>GSHMPAPHGGILQDLIARDALKKNELLSEAQSSDILVWNLTPRQLCDIELILNGGFSPLTGFLNENDYSSVVTDSRLADGTLWTIPITLDVDEAFANQIKPDTRIALFQDDEIPIAILTVQDVYKPNKTIEAEKVFRGDPEHPAISYLFNVAGDYYVGGSLEAIQLPQHYDYPGLRKTPAQLRLEFQSRQWDRVVAFQTRNPMHRAHRELTVRAAREANAKVLIHPVVGLTKPGDIDHHTRVRVYQEIIKRYPNGIAFLSLLPLAMRMSGD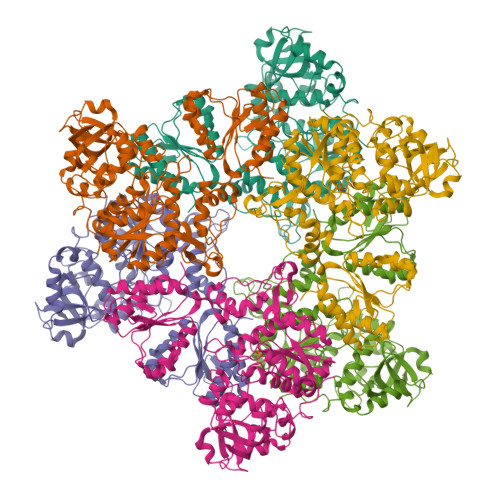REAVWHAIIRKNYGASHFIVGRDHAGPGKNSKGVDFYGPYDAQELVESYKHELDIEVVPFRMVTYLPDEDRYAPIDQIDTTKTRTLNISGTELRRRLRVGGEIPEWFSYPEVVKILRESNPPRPKQGFSIVLGNSLTVSREQLSIALLSTFLQFGGGRYYKIFEHNNKTELLSLIQDFIGSGSGLIIPNQWEDDKDSVVGKQNVYLLDTSSSADIQLESADEPISHIVQKVVLFLEDNGFFVF[3x]> MPPQLHNGLDFSAKVIQGSLDSLPQEVRKFVEGNAQLCQPEYIHICDGSEEEYGRLLAHMQEEGVIRKLKKYDNCWLALTDPRDVARIDSKTVIITQEQRDTVPIPKSGQSQLGRWMSEEDFEKAFNARFPGCMKGRTMYVIPFSMGPLGSPLAKIGIELTDSPYVVASMRIMTRMGTSVLEALGDGEFIKCLHSVGCPLPLKKPLVNNWACNPELTLIAHLPDRREIISFGSGYGGNSLLGKKCFALRIASRLAKEEGWLAEHMLILGITNPEGKKKYLAAAFPSACGKTNLAMMNPTLPGWKVECVGDDIAWMKFDAQGNLRAINPENGFFGVAPGTSVKTNPNAIKTIQKNTIFTNVAETSDGGVYWEGIDEPLAPGVTITSWKNKEWRPQDEEPCAHPNSRFCTPASQCPIIDPAWESPEGVPIE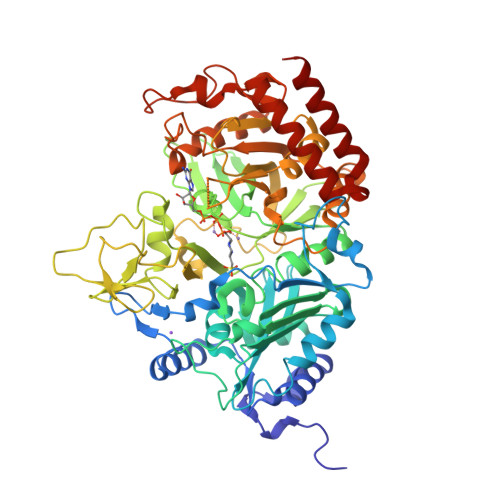GIIFGGRRPAGVPLVYEALSWQHGVFVGAAMRSEATAAAEHKGKVIMHDPFAMRPFFGYNFGKYLAHWLSMAHRPAAKLPKIFHVNWFRKDKNGKFLWPGFGENSRVLEWMFGRIEGEDSAKLTPIGYVPKEDALNLKGLGDVNVEELFGISKEFWEKEVEEIDKYLEDQVNADLPYEIERELRALKQRISQM>GIDPFTMTPSEDFVVTDRGGIVENSHRVHAAVVDAKGRLLYALGNPTRMTLARSAAKPAQALAILETEGVAGYGFDDADIALMCAAHSSEDRHIARTRAMLSKIKAEEADLRCGGHPSLSEMVNRSWIKQDFIPTAVCSNCSGKHVGMLAGARAIGAGTDGYHLPDHPMQGRVKRTVAELCDLDAGDVEWGTDGCNLPTPAFPLDRLGRIYAKLASAADGSDAGEGQSTRCAALAHIFRAMARHPEMVAGEGRYCTMLMRAFDGALVGKLGADASYAIGVRASDATRQLGTDGALGISVKIEDGNLEMLYAVVTELLERLGIGSPDVRSQLASFHHPQRVNTMGVTTGGVSFPFKLRGSKSNVDDPRLAAVAR[4x]

The ReAV enzyme from Rhizobium etli, a representative of Class 3 L-asparaginases, is sequentially and structurally different from other known L-asparaginases. Asparaginases (EC 3.5.1.1) catalyze the hydrolysis of L-asparagine, generating L-aspartate and ammonia. ReAV is a homodimeric protein, with each subunit containing a highly specific zinc-binding site created by two cysteines, a lysine, and a water molecule. Two Ser-Lys tandems (Ser48-Lys51, Ser80-Lys263) are located in the close proximity of the metal binding site, with Ser48 hypothesized to be the catalytic nucleophile.

The introduction of alanine at position 80 resulted in minor structural rearrangements of the protein in the active site area, which were nearly identical in the four protein chains. The S80A substitution affected the hydration pattern of Ser48, which is no longer surrounded by the triad of closely spaced water molecules. The Oγ atom of Ser48 is H-bonded to the Nζ atom of Lys51 and two water molecules, resembling two water molecules of the typical “triangle”. The Nζ atom of Lys263 is no longer able to interact with the Oγ atom of Ser80, but it continues to form H-bonds with the neighboring water molecule and the carbonyl oxygen of Leu264. The fully occupied Zn2+ binding site is conserved in the mutant structure. As observed in the S48A and K51A mutants, a sulfate ion from the crystallization solution is located at full occupancy near the metal binding site, forming H-bonds with the Nη atom of Arg47 and the main-chain N atoms of Gly188 and Cys189, as well as with several water molecules, one of which belongs to the metal coordination sphere. The side chain of Cys249 is most likely oxidized and was modeled as cysteinesulfinic acid. Another serine residue, namely Ser80 from the second Ser-Lys tandem, is an important hub for the H-bond network in the active site, interacting inter alia with the Ser48 nucleophile, to the point of forcing a non-planar configuration of the Ala79-Ser80 peptide bond. The S80A mutation turned the protein activity off, as the proton shuttling network could not function properly. Furthermore, the mutation led to protein aggregation, suggesting an additional role of Ser80 in maintaining the structural integrity of the protein.> CSSPKPDAEEQGVPVSPTASDPALLAEIRQSLDATKGLTSVHVAVRTTGKVDSLLGITSADVDVRANPLAAKGVCTYNDEQGVPFRVQGDNISVKLFDDWSNLGSISELSTSRVLDPAAGVTQLLSGVTNLQAQGTEVIDGISTTKITGTIP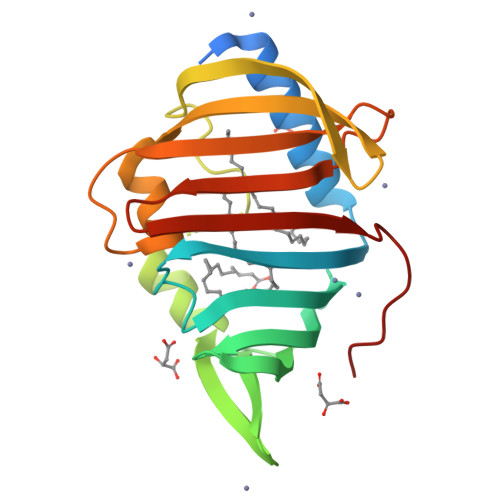ASSVKMLDPGAKSARPATVWIAQDGSHHLVRASIDLGSGSIQLTQSKWNEPVNVD>QGHVGDHDSHEVMQRLDALLPTLRERAQETEDLRRIPDDSMKALQETGFFRLLQPEQWGGYQADPVLFYSAVRKIASACGSTGWVSSIIGVHNWHLALFSQQAQEDVWGNDTDVRISSSYAPMGAGQVVDGGYTVNGAWAWSSGCDHASWAVLGGPVIKDGRPVDFVSFLIPREDYRIDDVWNVVGLRGTGSNTVVVEDVFVPTHRVLSFKAMSNLTAPGLERNTAPVYKMPWGTIHPTTISAPIVG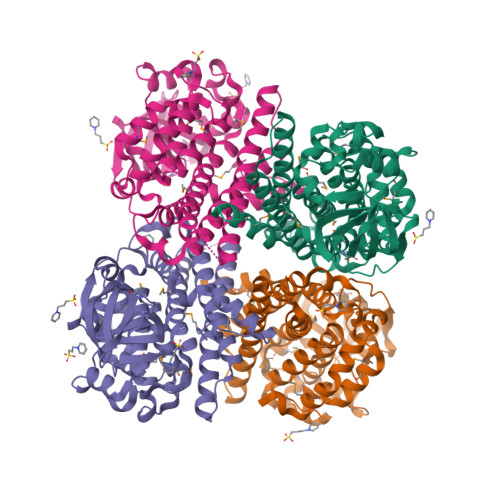MAYGAYDAHVEHQGKRVRAAFAGEKAKDDPFAKVRIAEASSDIDAAWRQLSGNVADEYALLVAGEEVPFELRLRARRDQVRATGRAISSIDKLFESSGATALANGTPLQRFWRDAHAGRVHAANDPERAYVMYGTGEFGLPITDTMV[4x]> AAWLPFARAAAIGWMPVANCPMPLAPADKNKRQDELIVLNVSGRRFQTWRTTLERYPDTLLGSTEKEFFFNEDTKEYFFDRDPEVFRCVLNFYRTGKLHYPRYEC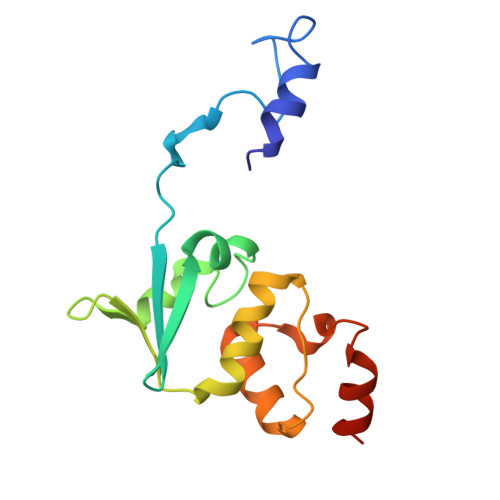ISAYDDELAFYGILPEIIGDCCYEEYKDRKRENAE> MSQEIRQNEKISYRIEGPFFIIHLMNPDNLNALEGEDYIYLGELLELADRNRDVYFTIIQSSGRFFSSGADFKGIAKAQGDDTNKYPSETSKWVSNFVARNVYVTDAFIKHSKVLICCLNGPAIGLSAALVALCDIVYSINDKVYLLYPFANLGLITEGGTTVSLPLKFGTNTTYECLMFNKPFKYDIMCENGFISKNFNMPSSNAEAFNAKVLEELREKVKGLYLPSCLGMKKLLKSNHIDAFNKANSVEVNESLKYWVDGEPLKRFRQLGSKQRKHRL;> ADVGSCSVGNNPLAQLHKHTQQNKSLQFNQKNNGRLNESPLQGTNKPGISEAFISNVNAISQENMANMQRFINGEPLIDDKRRMEIGPSSGRLPPFSNVHSLQTSANPTQIKGVNDISHWSQEFQGSNSIQNRNADTGNSEKAWQRGSTTASSRFQYPNTMMNNYAYASMNSLSGSRLQSPAFMNQQQSGRSKEGVNEQEQQPWTDQFEKLEKEVSENLDINDEIEKEENVSEVEQNKPETVEKEEGVYGDQYQSDFQEVWDSIHKDAEEVLPSELVN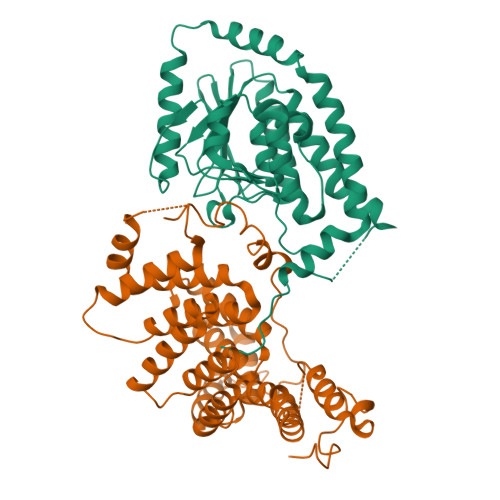DDLNLGEDYLKYLGGRVNGNIEYAFQSNNEYFNNPNAYKIGCLLMENGAKLSEAALAFEAAVKEKPDHVDAWLRLGLVQTQNEKELNGISALEECLKLDPKNLEAMKTLAISYINEGYDMSAFTMLDKWAETKYPEIWSRIKQQDDKFQKEKGFTHIDMNAHITKQFLQLANNLSTIDPEIQLCLGLLFYTKDDFDKTIDCFESALRVNPNDELMWNRLGASLANSNRSEEAIQAYHRALQLKPSFVRARYNLAVSSMNIGCFKEAAGYLLSVLSMHEVNTNNKKGDVGSLLNTYNDTVIETLKRVFIAMNRDDLLQEVKPGMDLKRFKGEFSF methyl 3-(5-bromo-2,4-dioxo-3,4-dihydropyrimidin-1(2H)-yl)-L-alaninate | C8 H10 Br N3 O4 | 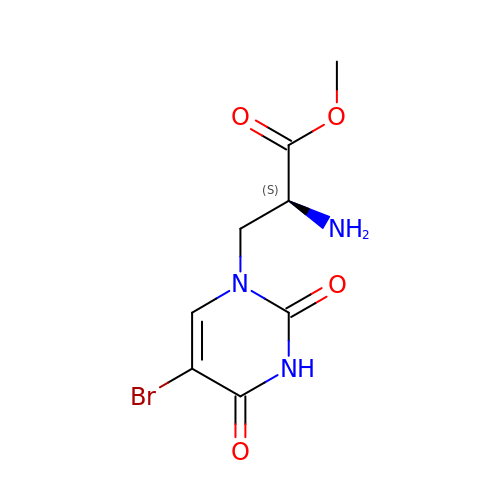SWCNOWRHWSFLMA-YFKPBYRVSA-N9R,13R-12-OXOPHYTODIENOIC 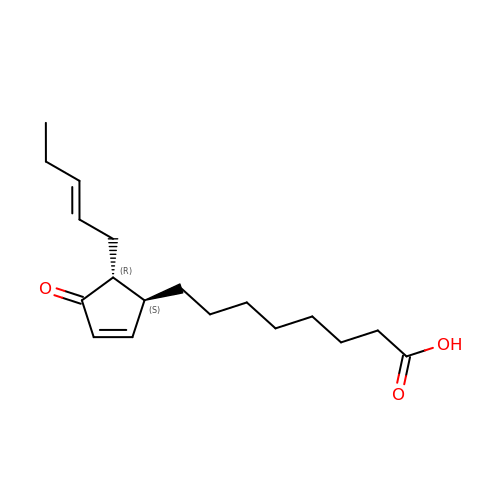ACID | C18 H28 O3 | PMTMAFAPLCGXGK-HZPDHXFCSA-N> MAAPLVLVLVVAVTVRAALFRSSLAEFISERVEVVSPLSSWKRVVEGLSLLDLGVSPYSGAVFHETPLIIYLFHFLIDY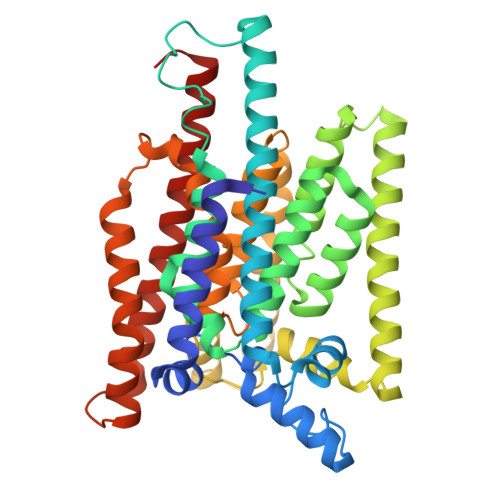AELVFMITDALTAIALYFAIQDFNKVVFKKQKLLLELDQYAPDVAELIRTPMEMRYIPLKVALFYLLNPYTILSCVAKSTCAINNTLIAFFILTTIKGSAFLSAIFLALATYQSLYPLTLFVPGLLYLLQRQYIPVKMKSKAFWIFSWEYAMMYVGSLVVIICLSFFLLSSWDFIPAVYGFILSVPDLTPNIGLFWYFFAEMFEHFSLFFVCVFQINVFFYTIPLAIKLKEHPIFFMFIQIAVIAIFKSYPTVGDVALYMAFFPVWNHLYRFLRNIFVLTCIIIVCSLLFPVLWHLWIYAGSANSNFFYAITLTFNVGQILLISDYFYAFLRREYYLTHGL The tripartite ATP-independent periplasmic (TRAP) transporters use an extra cytoplasmic substrate binding protein (SBP) to transport a wide variety of substrates in bacteria and archaea. The SBP (commonly referred to as the P-domain in TRAP transporters) is a soluble protein that freely diffuses in the periplasm of Gram-negative bacteria or is associated with the cell membrane in Gram-positive bacteria and archaea. It scavenges substrate molecules and delivers them to the membrane transporter. Since then, many more structures have been determined, confirming the general architecture of the P-domain as two globular lobes connected by a long backbone helix (red).

We searched the structural model of the HiSiaPQM complex for sites where the different domains can be locked in a given conformational state by intra-chain disulfide bonds. As shown in Fig. 1 (right), we selected two pairs of residues in HiSiaP (S44C/S171C and S15C/A194C) and named the two constructs HiSiaP CLOSED #1 and HiSiaP CLOSED #2, respectively. For both constructs, the thiol groups of the introduced cysteines would likely be in close proximity in the substrate-bound state, and the formation of a disulfide bond would therefore be expected to lock the SBP in this conformation. To verify that the disulfide-linked SBPs had the expected structure, we set up crystallization experiments of the H2O2-treated HiSiaP CLOSED #1/2 constructs. Heavily intergrown crystals of HiSiaP CLOSED #2 were obtained and single crystalline pieces could be broken off for diffraction data collection at the PETRA III synchrotron (DESY, Hamburg, Germany). A 1.9 Å data set (space group I222) was collected and the structure was solved by molecular replacement using the closed state of HiSiaP as a search model (PDB-ID: 3B506). A clear solution was found and inspection of the electron density map revealed density at the expected position of the disulfide bond and the sialic acid binding site, demonstrating that the disulfide bond had indeed been formed and the sialic acid molecule had been captured in its binding site. The two structures overlap with an r.m.s.d. value of 0.24 Å over 300 Cɑ atoms, and except for the introduced disulfide bond, there is no significant change between the backbone or side chain atoms of the two structures. We found that traces of a second conformation of C194 were visible in the electron density. The different position of the engineered cysteines along the edge of the substrate binding pocket explains the higher propensity of CLOSED #2 to spontaneously form a disulfide bond, even without an oxidation agent. Very clearly, HiSiaP CLOSED #2 preferably interacted with the IFS of HiSiaQM.

> GADYDLKFGMNAGTSCNEYKAAEMFAKEVKEKSQGKIEISLYPSSQLGDDRAMLKQLKDGSLDFTFAESARFQLFYPEAAVFALPYVISNYNVAQKALFDTEFGKDLIKKMDKDLGVTLLSQAYNGTRQTTSNRAINSIADMKGLKLRVPNAATNLAYAKYVGASPTPMAFSEVYLALQTNAVDGQENPLAAVQCQKFYEVQKFLAMTNHILNDQLYLVSNETYKELPEDLQKVVKDAAENAAKYHTKLFVDGEKDLVTFFEKQGVKITHPDLVPFKESMKPYYAEFVKQTGQKGESALKQIEAINPKGEA>SSPPVVDTVHGKVLGKFVSLEGFAQPVAIFLGIPFAKPPLGPLRFTPPQPAEPWSFVKNATSYPPMCTQDPKAGQLLSELFTNRKENIPLKLSEDCLYLNIYTPADLTKKNRLPVMVWIHGGGLMVGAASTYDGLALAAHENVVVVTIQYRLGIWGFFSTGDEHSRGNWGHLDQVAALRWVQDNIASFGGNPGSVTIFGESAGGESVSVLVLSPLAKNLFHRAISESGVALTSVLVKKGDVKPLAEQIAITAGCKTTTSAVMVHCLRQKTEEELLETTLKMKFLSLDLQGDPRESQPLLGTVIDGMLLLKTPEELQAERNFHTVPYMVGINKQEFGWLIPMLMSYPLSEGQLDQKTAMSLLWKSYPLVCIAKELIPEATEKYLGGTDDTVKKKDLFLDLIADVMFGVPSVIVARNHRDAGAPTYMYEFQYRPSFSSDMKPKTVIGDHGD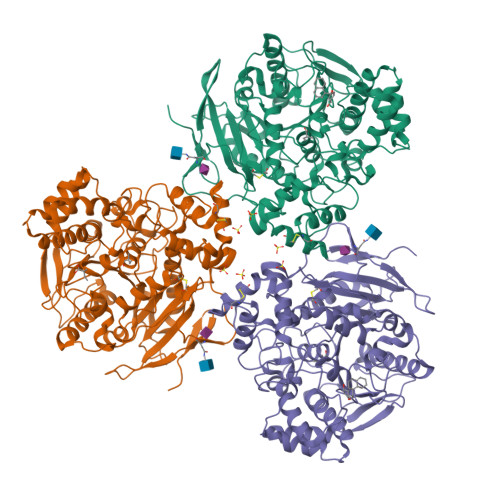ELFSVFGAPFLKEGASEEEIRLSKMVMKFWANFARNGNPNGEGLPHWPEYNQKEGYLQIGANTQAAQKLKDKEVAFWTNLFAK[3x]>MAEESRGQRGSGYGLGLSTRTQVTGYQFLARRTAMALTRWRVRMEIEPGRRQTLAVVASVSAALVICLGALLWSFISPSGQLNESPIIADRDSGALYVRVGDRLYPALNLASARLITGRPDNPHLVRSSQIATMPRGPLVGIPGAPSSFSPKSPPASSWLVCDTVATSSSIGSLQGVTVTVIDGTPDLTGHRQILSGSDAVVLRYGGDAWVIREGRRSRIEPTNRAVLLPLGLTPEQVSQARPMSRALFDALPVGPELLVPEVPNAGGPATFPGAPGPIGTVIVTPQISGPQQYSLVLGDGVQTLPPLVAQILQNAGSAGNTKPLTVEPSTLAKMPVVNRLDLSAYPDNPLEVVDIREHPSTCWWWERTAGENRARVRVVSGPTIPVAATEMNKVVSLVKADTSGRQADQVYFGPDHANFVAVTGNNPGAQTSESLWWVTDAGARFGVEDSKEARDALGLTLTPSLAPWVALRLLPQGPTLSRADALVEHDTLPMDMTPAELVVPK[6x];>MQRFGTGSSRSWCGRAGTATIAAVLLASGALTGLPPAYAISPPTIDPGALPPDGPPGPLAPMKQNAYCTEVGVLPGTDFQLQPKYMEMLNLNEAWQFGRGDGVKVAVIDTGVTPHPRLPRLIPGGDYVMAGGDGLSDCDAHGTLVASMIAAVPANGAVPLPSVPRRPVTIPTTETPPPPQTVTLSPVPPQTVTVIPAPPPEEGVPPGAPVPGPEPPPAPGPQPPAVDRGGGTVTVPSYSGGRKIAPIDNPRNPHPSAPSPALGPPPDAFSGIAPGVEIISIRQSSQAFGLKDPYTGDEDPQTAQKIDNVETMARAIVHAANMGASVINISDVMCMSARNVIDQRALGAAVHYAAVDKDAVIVAAAGDGSKKDCKQNPIFDPLQPDDPRAWNAVTTVVTPSWFHDYVLTVGAVDANGQPLSKMSIAGPWVSISAPGTDVVGLSPRDDGLINAIDGPDNSLLVPAGTSFSAAIVSGVAALVRAKFPELSAYQIINRLIHTARPPARGVDNQVGYGVVDPVAALTWDVPKGPAEPPKQLSAPLV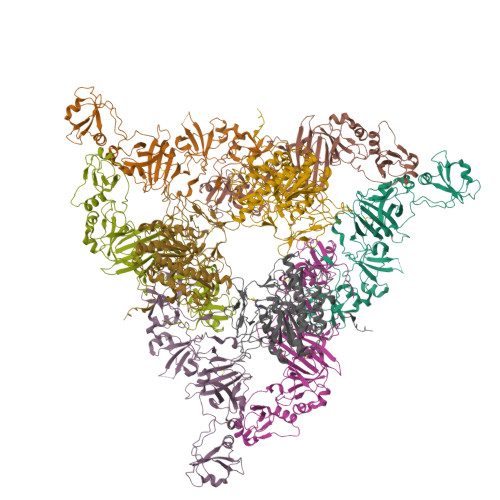VPQPPAPRDMVPIWVAAGGLAGALLIGGAVFGTATLMRRSRKQQ[3x]>[4x]MKDIKVEPAKGISYFTPAQETPAGTAANPQTSGKAIPKLFQPITIRGLTFQNRLGVSPMCQYSAEDGHMTDYHLAHLGGIAQRGPGLIMIE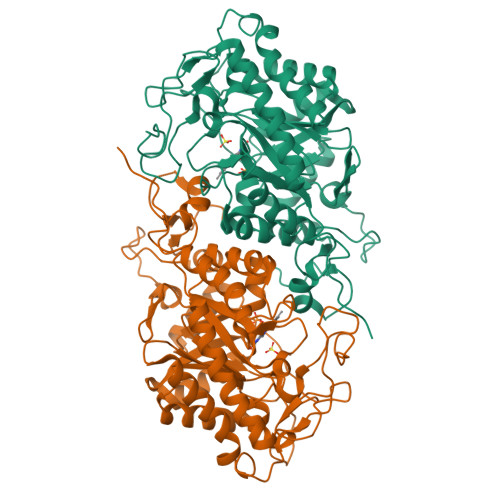ATAVQPEGRISPQDVGLWKDSQIAPIARVIEFAHSQGQKIGIQLAHAGRKASTTVPWMLNHGSIATENVGGWPDNVKGPSDIPFSETFPRPRAMTQDDIREFKEAWVAAAKRALVAGADFIEIHNAHGYLLASFLTPYANKRTDEYGGSFENRMRLPLKIAQLTRDTVGEHVPVFLRLSASDWLGSTSTETWDLQHAVRFAEALADQGAIDLVDVSSGGLHSSQEVKSGPGFQAPFGIAVKKAVGERMLVATVGHIRDGKLANRLLEEEGLDVVLVGRGFQKDPGLVWTFAQHLDVEVAMPGQIRWGFSKQGRRGTPFVDPSVYKPSVIEP PAK4 is a kinase with strong links to cellular transformation and cancer metastasis, as reviewed. We have shown that Cdc42 directly regulates PAK4 activity in mammalian cells through an auto-inhibitory domain (AID) that binds in a manner similar to pseudosubstrates. We have identified Inka1 as a potent vertebrate inhibitor of PAK4 with a Ki of ∼30 nM, which has a much higher affinity than the corresponding AID. The recombinant 38 amino acid ‘Inka box' (GST-iBox) is a potent of PAK4cat inhibitor in vitro but does not affect PAK1, suggesting Inka1 is a specific group II PAK30 inhibitor.

The C-terminal 31 amino acid of Inka1 (255–285) was able to induce crystals more efficiently than the Inka1 (166–203) when they are expressed as haemagglutinin (HA)-tagged proteins, although the iBox38 has a higher affinity in vitro. To confirm that these crystals indeed contain a 1:1 ratio of both components, we generated a single-chain Flag–iBox–PAK4cat construct as illustrated in Fig. 2c. To tackle the in-cellulo crystal structure of iBox–PAK4cat, intact monkey COS-7 cells that contained large single needle crystals (<5 μm in cross-section by 50–100 μm) were trypsinized to yield rounded cells in which large crystals could be easily observed (arrows). The X-ray structure of these in-cellulo crystals provided us with a number of important insights: under cellular conditions, PAK4cat adopts a typical ‘closed' active kinase conformation that includes ATP bound to two magnesium ions. As we expected, the activation (A) loop Ser474 is phosphorylated and the central region of the iBox is packed against the kinase through both main-chain and side-chain interactions. On the basis of these experiments, we hypothesize that Inka1 stabilizes the ATP-bound crystallization-competent conformation of the kinase domain by preventing ATP hydrolysis through binding tightly in the cleft between the N- and C-lobes. Inspection of the crystal packing revealed that the crystal is formed by only two types of contacts, both of which are between PAK4cat units. In the in-cellulo crystals one set of crystal contacts is formed by the interaction between neighbouring N-lobes that involves the two helices from one N-lobe interacting with the β-sheet of the adjacent N-lobe, an interaction area of 768 Å2. The second set of contacts lies at the threefold axis mediated by the PAK4cat C-lobes involving primarily hydrophobic residues; each C-lobe contributes 576 Å2 to this crystal contact. Remarkably, the iBox is not involved in crystal contacts and is exposed to the large 80-Å-diameter central solvent channels that run the length of the crystals.

> MDYKDDDDKSGSEAEDWTAALLNRGRSRQPLVLGDNCFADLVHNWMELPEEFPAAPAVPGPPGPRSPQREPQRVSHEQFRAALQLVVDPGDPRSYLDNFIKIGEGSTGIVCIATVRSSGKLVAVKKMDLRKQQRRELLFNEVVIMRDYQHENVVEMYNSYLVGDELWVVMEFLEGGALTDIVTHTRMNEEQIAAVCLAVLQALSVLHAQGVIHRDIKSDSILLTHDGRVKLSDFGFCAQVSKEVPRRKSLVGTPYWMAPELISRLPYGPEVDIWSLGIMVIEMVDGEPPYFNEPPLKAMKMIRDNLPPRLKNLHKVSPSLKGFLDRLLVRDPAQRATAAELLKHPFLAKAGPPASIVPLMRQNRTR5-chloranyl-3~{H}-1,3-benzoxazole-2-thione | C7 H4 Cl N O S | 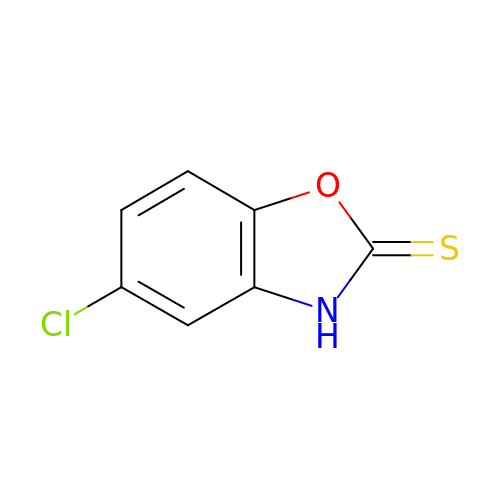BOBIZYYFYLLRAH-UHFFFAOYSA-N3,4-dinitrophenol | C6 H4 N2 O5 | 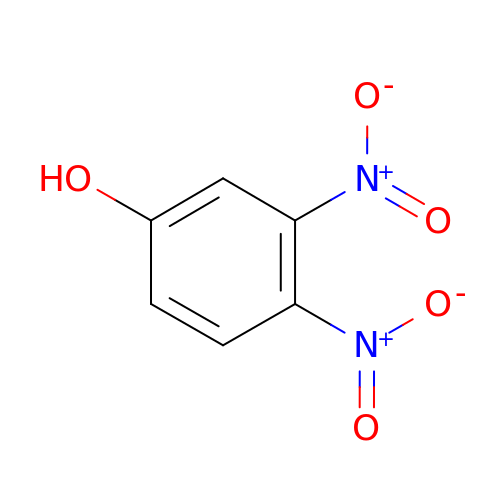AKLOLDQYWQAREW-UHFFFAOYSA-N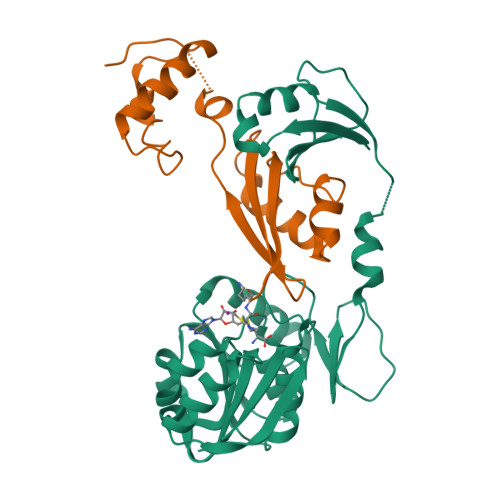>[3x]MWVYRLKGTLEALDPILPGLFDGGARGLWEREGEVWAFFPAPVDLPYEGVWEEVGDEDWLEAWRRDLKPALAPPFVVLAPWHTWEGAEIPLVIEPGMAFGTGHHETTRLALKALARHLRPGDKVLDLGTGSGVLAIAAEKLGGKALGVDIDPMVLPQAEANAKRNGVRPRFLEGSLEAALPFGPFDLLVANLYAELHAALAPRYREALVPGGRALLTGILKDRAPLVREAMAGAGFRPLEEAAEGEWVLLAYGR;>[3x]KKVVAVVKLQLPAGKATPAPPVGPALGQHGANIMEFVAAFNAATANMGDAIVPVEITIYADRSFTFVTKTPPASYLIRKAAGLEKGAHKPGREKVGRITWEQVLEIAKQKMPDLNTTDLEAAARMIAGSARSMGVEVVGAPEVKDA> SDSISVDALVQEFFAQQSLKILPQAPFGDAVNQ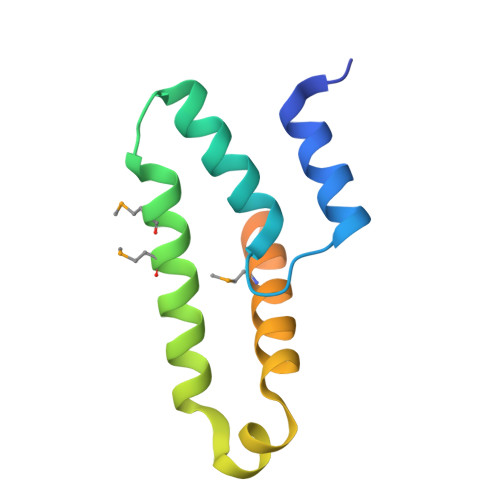FVSKDDKHAVEMFVMDSLSSQVRGLLQLDDDKINEGLDSHIEDFRKVMEKNFLSGQQKQAQRRRRFKEKHHHHHH> GPLGSETQAGIKEEIRRQEFLLNSLHRDLQGGIKDLSKESRMWEVLRILTALRRKLRE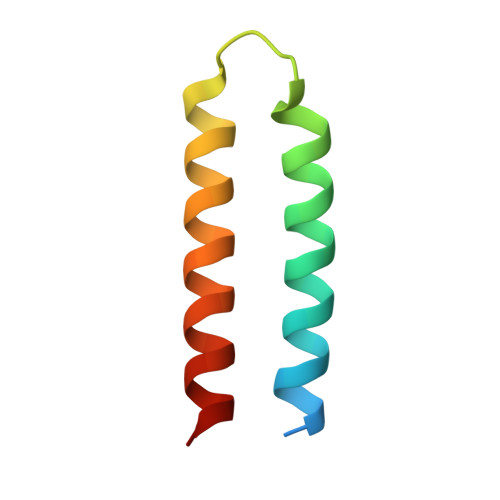A The potent neurotoxic venom of the black widow spider contains a cocktail of seven phylum-specific latrotoxins (LTXs), but only one, α-LTX, targets vertebrates. This 130 kDa toxin binds to receptors at presynaptic nerve terminals and triggers a massive release of neurotransmitters. Each monomer is composed of an N-terminal four-helix connector domain (CD; residues E21–D115), a central helical bundle domain (HBD; residues S116–K350), a short β-sheet plug domain (PD; residues Q351–D453) and a C-terminal tail of 22 ARs (ARD; residues I454–G1195).

The architecture of each subunit of state 1 has a characteristic G-shape and is similar to that of the soluble α-LCT monomer and the δ-LIT dimer19. The four HBDs form the core of the tetramer with a central ~12–15 Å channel and the ARDs extend to the periphery, in a four-bladed windmill-like assembly. The tetramer in the prepore state is assembled by stronger interactions between the PD of one monomer and ARs 1–6 of the clockwise neighboring monomer and is further stabilized by weaker interactions between the HBDs and PDs of neighboring monomers. Interestingly, in the prepore state, the CD is sandwiched in a pocket between the three other domains of the monomer and completely avoids interactions with neighboring monomers. We observe significant movements of the HBDs and ARDs relative to each other, inducing conformation heterogeneities and symmetry breaks in the potential four-fold symmetry. The prepore displays a high degree of conformational flexibility in the curvature and/or relative orientation of different subunits and domains, resulting in “breathing motions” of the central channel. Moreover, in the prepore state, the helices of the N-terminal CD are tightly packed and protected within a groove formed between the HBD and the ARD-tail, with helices α1–α3 being fragmented, but stabilized by a conserved disulfide bond. Direct comparison of the cryo-EM structure of the N-terminal helices α1–α3 in the prepore state with their AlphaFold2 prediction in the pore state suggests that these helices undergo dramatic conformational changes to assemble the TMD: In the prepore state, α1–α3 are isolated within each monomer, with a distance of ~60–80 Å to each other, and are bent into a total of five shorter sub helices (α1a, α1b, α2, α3a, and α3b). A stepwise assembly of the tetrameric prepore can easily be rationalized by the involved subunit interactions, which are almost exclusively formed between the PD of one monomer with the AR domain of the clockwise neighboring monomer. The tetrameric prepore is well resolved in this region and shows that the introduced VPRG residues are placed N-terminal of the last β-sheet (β7) of the PD domain, disturbing the crucial intermolecular oligomerization site between PD and neighboring ARD.

>MISVGEIMERANHSLVRMRREGEDLTLEEKAEICSELELQQKYVDIASNIIGDLSSLPIAGKIAGTIAAAAMTATHVASGRLDIEQTLLGCSDLPFDQIKEVLENRFNEIDRKLDSHSAALEEITKLVEKSISVVEKTRKQMNKRFDEVMKSIQDAKVSPIISKINNFARYFDTEKERIRGLKLNDYILKLEEPNGILLHFKESRTPTDDSLQAPLFSIIEEGYAVPKSIDDELAFKVLYALLYGTQTYVSVMFFLLEQYSFLANHYYEKGYLEKYDEYFNSLNNVFLDFKSSLVGTGTSNNEGLLDRVLQVLMTVKNSEFLGLEKNGVDEMLNEKINLFNKIKEEIEGKQKMTLSETPENFAQISFDKDITTPIGDWRDGREVRYAVQYASETLFSKISHWSDPVSVREKACPTLRMPVDQTRRNVLVFRKFDSSKPQLVGEITPYLSNFIDIDRDLYNAASNPDSAVGFKEFTKLNYDGANIRATFDHGRTVFHAAAKSGNDKIMFGLTFLAKSTELNQPDKKGYTPIHVAADSGNAGIVNLLIQRGVSINSKTYHFLQTPLHLAAQRGFVTTFQRLMESPEININERDKDGFTPLHYAIRGGERILEAFLNQISIDVNAKSNTGLTPFHLAIIKNDWPVASTLLGSKKVDINAVDENNITALHYAAILGYLETTKQLINLKEINANVVSSPGLLSALHYAILYKHDDVASFLMRSSNVNVNLKALGGITPLHLAVIQGRKQILSLMFDIGVNIEQKTDEKYTPLHLAAMSKYPELIQILLDQGSNFEAKTNSGATPLHLATFKGKSQAALILLNNEVNWRDTDENGQMPIHGAAMTGLLDVAQAIISIDATVVDIEDKNSDTPLNLAAQNSHIDVIKYFIDQGADINTRNKKGLAPLLAFSKKGNLDMVKYLFDKNANVYIADNDGMNFFYYAVQNGHLNIVKYAMSEKDKFEWSNTDNNRRDECPNEECAISHFAVCDAVQFDRIEIVKYFVGTLGNFAICGPLHQAARYGHLDIVKYLVEEEFLSVDGSKTDTPLCYASENGHFTVVQYLVSNGAKVNHDCGNGMTAIDKAITKNHLQVVQFLAANGVDFRRKNSRGTTPFLTAVAENALHIAEYLIREKRQDININEQNVDKDTALHLAVYYKNLQMIKLLIKYGIDVTIRNAYDKTALDIAIDAKFSNIVEYLKTKSGKFRREYKSSYGERSLLQTNQISNFIDRKNIEHDHPLFINADNESSELFSKTASNIDVIGTLLLIDVLIRYFSKQGYISKESDSASDGITQAAALSITEKFEDVLNSLHNESAKEQVDLAEVHGKVYAALKSGRNSQIHQILCSSLNSISTLKPEDMEKLESVIMNSHSSVSLPEVTDSANEAYGETLHLFGESCLHSDGILTKKLM[4x]> VVGGDECNINEHPFLVALYTSASSTIHCAGALINREWVLTAAHCDRRNIRIKLGMHSKNIRNEDEQIRVPRGKYFCLNTKFPNGLDKDIMLIRLRRPVTYSTHIAPVSLPSRSRGVGSRCRIMGWGKISTTTYPDVPHCTNIFIVKHKWCEPLYPWVPADSRTLCAGILKGGRDTCHGDSGGPLICNGEMHGIVAGGSEPCGQHLKPAVYTKVFDYNNWIQSIIA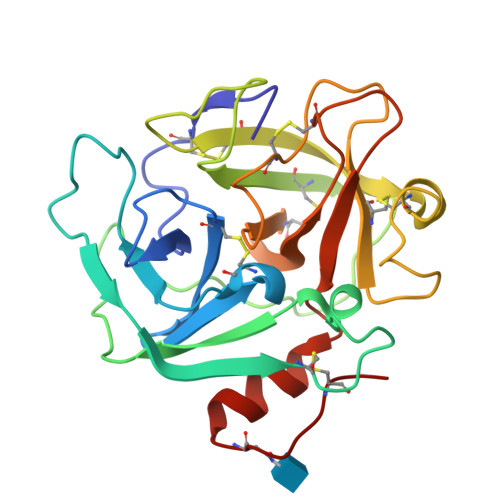GNRTVTCPP>MEVHMLSKDNKKSIRKTLEQRRGEYAYYVIKEVADLNDKQLEEKYASLVKKAPVMILSNGLLQTLAFLLAKAETSPEKANQILSRVNEYPPRFIEKLGNDKDEHLLLYLHIVYWLRENVDRNIDVKTLLSQDYSKVLWATK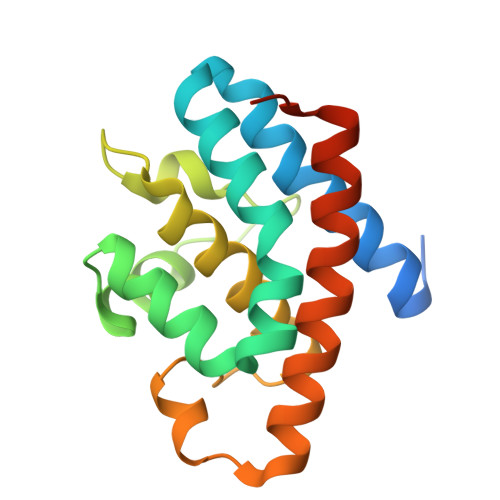EAIALLNWMRRFAVAMLKEEGKENEGSS[2x]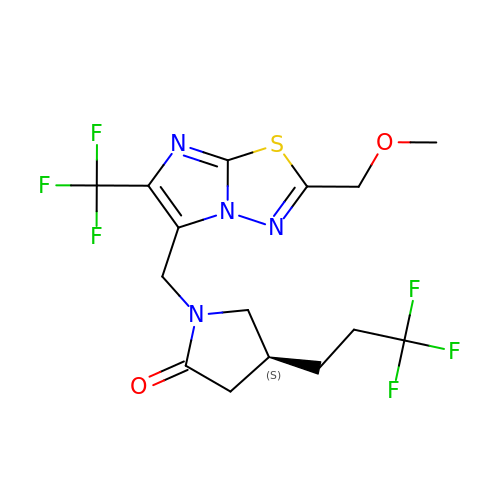(4S)-1-{[(4S)-2-(methoxymethyl)-6-(trifluoromethyl)imidazo[2,1-b][1,3,4]thiadiazol-5-yl]methyl}-4-(3,3,3-trifluoropropyl)pyrrolidin-2-one | C15 H16 F6 N4 O2 S | WZUOWEYSJYNQFH-QMMMGPOBSA-N>[2x]MRFFLSPPHMGGNELKYIEEVFKSNYIAPLGEFVNRFEQSVKDYSKSENALALN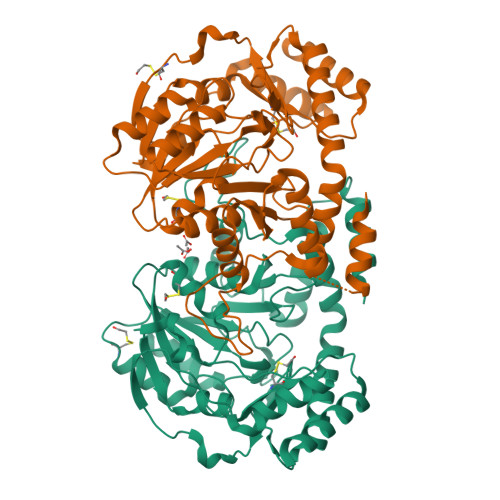SATAALHLALRVAGVKQDDIVLASSFTFIASVAPICYLKAKPVFIDCDETYNIDVDLLKLAIKECEKKPKALILTHLYGNAAKMDEIVEICKENDIVLIEDAAEALGSFYKNKALGTFGEFGVYSYNGNKIITTSGGGMLIGKNKEKIEKARFYSTQARENCLHYEHLDYGYNYRLSNVLGAIGVAQMEVLEQRVLKKREIYEWYKEFLGEYFSFLDELENSRSNRWLSTALINFDKNELNACQKDINISQKNITLHPKISKLIEDLKNKQIETRPLWKAMHTQEVFKGAKAYLNGNSELFFQKGICLPSGTAMSKDDVYEISKLILKSIKAGSHHHHHH>SMMQKLVVTRLSPNFREAVTLSRDCPVPLPGDGDLLVRNRFVGVNASDINYSAGRYDPSVKPPFDIGFEGIGEVVALGLSASARYTVGQAVAYMAPGSFAEYTVVPASIATPVPSVKPEYLTLLVSGTTAYISLKELGGLSEGKKVLVTAAAGGTGQFAMQLSKKAKCHVIGTCSSDEKSAFLKSLGCDRPINYKTEPVGTVLKQEYPEGVDVVYESVGGAMFDLAVDALATKGRLIVIGFISGYQTPTGLSPVKAGTLPAKLLKKSASVQGFFLNHYLSKYQAAMSHLLEMCVSGDLVCEVDLGDLSPEGRFTG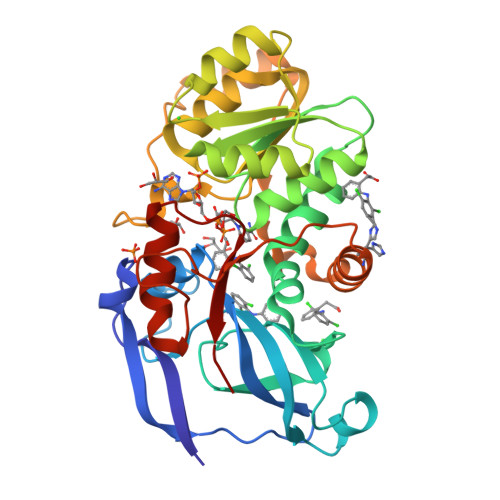LESIFRAVNYMYMGKNTGKIVVELPH[2x]> IVGGYTCGANTVPYQVSLNSGYHFCGGSLINSQWVVSAAHCYKSGIQVRLGEDNINVVEGNEQFISASKSIVHPSYNSNTLNNDIMLIKLKSAASLNSRVASVSLPTSCASAGTQCLISGWGNTKSSGTSYPDVLKCLKAPILSDSSCKSAYPGQITSNMFCAGYLEGGKDSCQGDSGGPVVCAGKLQGIVSWGSGCAQKNKPGVYTKVC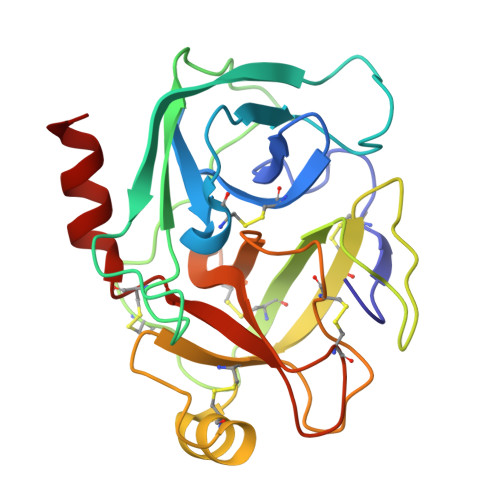NYVSWIKQTIASN>ASGLVASNLNLKPGESLRVRGEVAPDAKSFVLNLGKDSNNLSLHFNPRFNAHGDANTIVSNSKDGGAWGTEQREAVFPFQPGSVAEV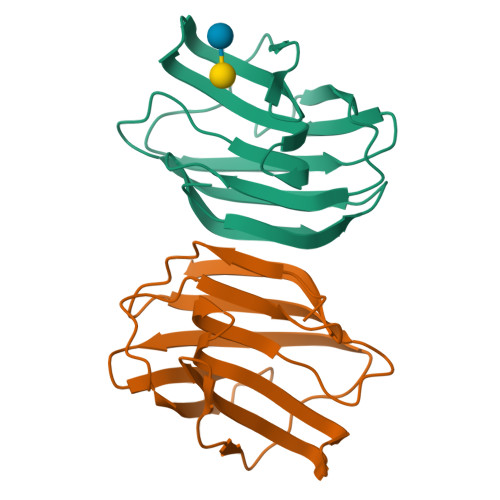SITFDQANLTVKLPDGYEFKFPNRLNLEAINYMAADGDFKIKSVAFD[2x]> AASDSAQLKSAREDIKELLKTKFCHPIMVRLGWHDAGTYNKNIEEWPQRGGANGSLRFDVELKHGANAGLVNALNLLKPIKDKYSGVTYADLFQLASATAIEEAGGPKIPMKYGRVDVTEPEQCPEEGRLPDAGPPSPAQHLRDVFYRMGLNDKEIVALSGAHTLGRSRPDRSGWGKPETKYTKDGPGAPGGQSWTAQWLKFDNSYFKDIKERRDEDLLVLPTDAALFEDPSFKVYA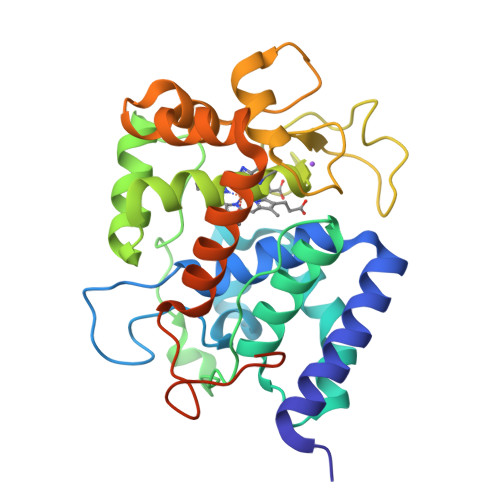EKYAADPEAFFKDYAEAHAKLSNLGAKFGPAEGFSLEGSPAGAAPEKFVAAKYSTGKD1-Naphthalenepentanoic acid | C15 H16 O2 | 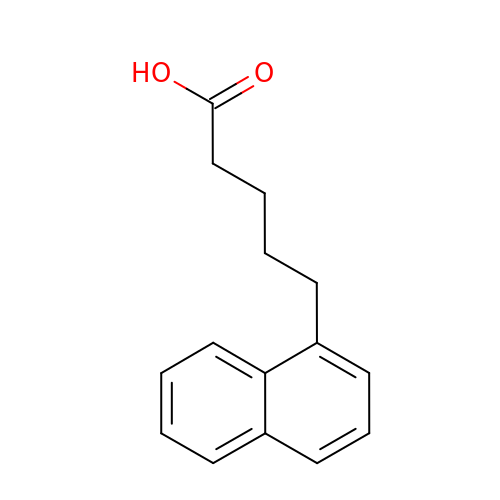MBQDHVLINYDJHO-UHFFFAOYSA-N>[6x]MLPKLVITHRVHEEILQLLAPHCELITNQTDSTLTREEILRRCRDAQAMMAFMPDRVDADFLQACPELRVIGCALKGFDNFDVDACTARGVWLTFVPDLLTVPTAELAIGLAVGLGRH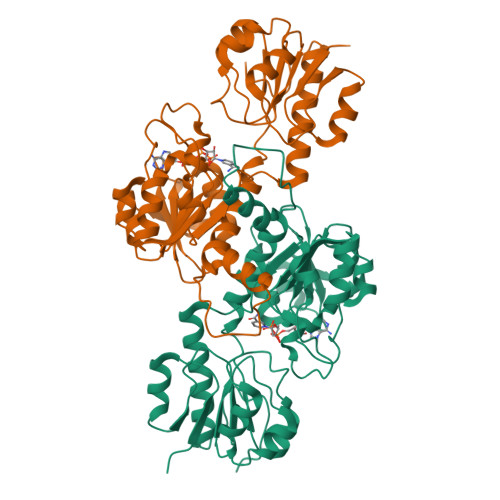LRAADAFVRSGQFRGWQPRFYGTGLDNATVGFLGMGAIGLAMADRLQGWGATLQYHARKALDTQTEQRLGLRQVACSELFASSDFILLALPLNADTLHLVNAELLALVRPGALLVNPCRGSVVDEAAVLAALERGQLGGYAADVFEMEDWARADRPQQIDPALLAHPNTLFTPHIGSAVRAVRLEIERCAAQNILQALAGERPINAVNRLPKAN> RKAK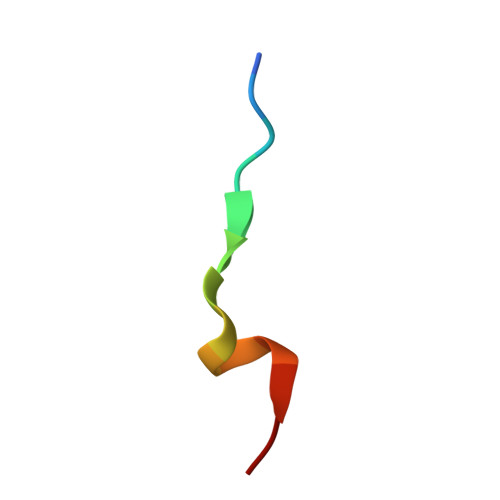LLPMEEALLP>[2x]MMCLKLNLLDHVFANPFMNAAGVLCSTEEDLRCMTASSSGALVSKSCTSAPRDGNPEPRYMAFPLGSINSMGLPNLGFDFYLKYASDLHDYSKKPLFLSISGLSVEENVAMVRRLAPVAQEKGVLLELNLS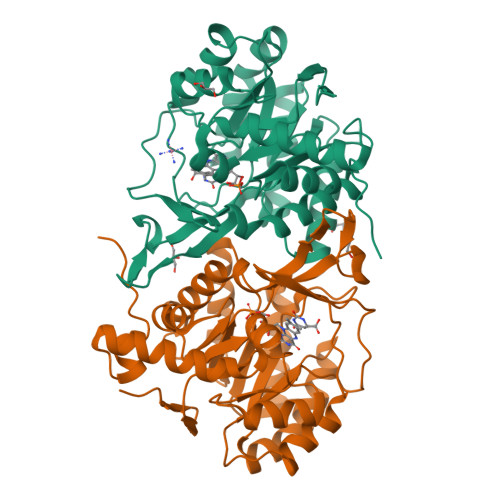CPNVPGKPQVAYDFEAMRTYLQQVSLAYGLPFGVKMPPYFDIAHFDTAAAVLNEFPLVKFVTCVNSVGNGLVIDAESESVVIKPKQGFGGLGGKYILPTALANVNAFYRRCPDKLVFGCGGVYSGEDAFLHILAGASMVQVGTALQEEGPGIFTRLEDELLEIMARKGYRTLEEFRGRVKTIE> GSRFVVEKNNLKVTSPDSIKGIYECAIGNFGVPQYGGTLVGTVVYPKSNQKACKSYSDFDISFKSKPGRLPTFVLI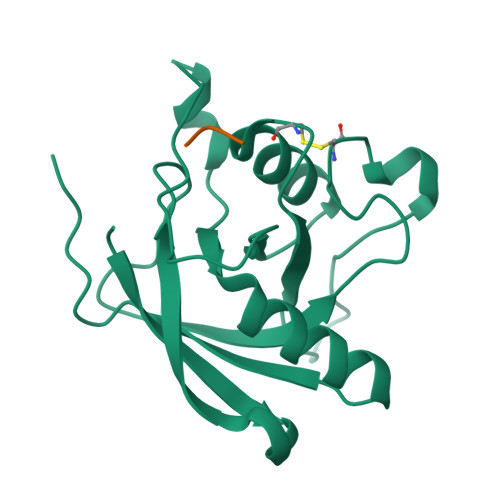DRGDCYFTLKAWIAQQAGAAAILVADSKAEPLITMDTPEEDKSDADYLQNITIPSALITKTLGDSIKSALSGGDMVNMKLDWTESVPHP;> ADSNPIRPVT> GSDNAEKGKVSNDDASVDFVAEPVKLPENQTRVAFFYDRAVPIGMLRPGQNIE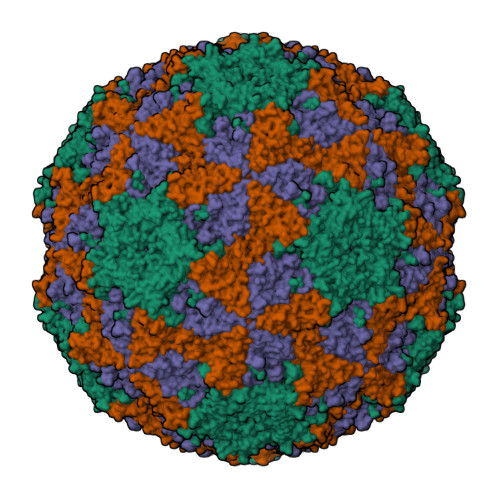STFVYQENDLRLNCLLLTPLPSFCPDSTSGPVKTKAPVQWRWVRSGGTTNFPLMTKQDYAFLCFSPFTYYKCDLEVTVSALGTDTVASVLRWAPTGAPADVTDQLIGYTPSLGETRNPHMWLVGAGNTQISFVVPYNSPLSVLPAAWFNGWSDFGNTKDFGVAPNADFGRLWIQGNTSASVRIRYKKMKVFCPRPTLFFPWPVSTRSKINADNPVPILELE;> DQNTEEMENLSDRVASDKAGNSATNTQSTVGRLCGYGEAHHGEHPASCADTATDKVLAAERYYTIDLASWTTTQEAFSHIRIPLPHVLAGEDGGVFGATLRRHYLCKTGWRVQVQCNASQFHAGSLLVFMAPEFYTGKGTKTGDMEPTDPFTMDTTWRAPQGAPTGYRYDSRTGFFAMNHQNQWQWTVYPHQILNLRTNTTVDLEVPYVNIAPTSSWTQHANWTLVVAVFSPLQYASGSSSDVQITASIQPVNPVFNGLRHETVIAQ;> SPIAVTVREHKGCFYSTNPDTTVPIYGKTISTPNDYMCGEFSDLLELCKLPTFLGNPNSNNKRYPYFSATNSVPTTSLVDYQVALSCSCMCNSMLAAVARNFNQYRGSLNFLFVFTGAAMVKGKFLIAYTPPGAGKPTTRDQAMQATYAIWDLGLNSSFVFTAPFISPTHYRQTSYTSATIASVDGWVTVWQLTPLTYPSGTPVNSDILTLVSAGDDFTLRMPISPTKWVPQGSDN;> GNASSSDKSNSQSSGNEGVIINNFYSNQYQNSIDLSASGGNAGDAPQNNGQLSNILGGAANAFATMAPLLL> MYVFRFHISSFHSFLVNFLQPSRGVGEPSRLLHHLETHPSYMRRVTSTAVHRTVSSVLSPALLPSFNGTLLLSVCFASCSAAPVRNLYKRLGLDHKATSEEVKAAYRQRALECHPDVVDDNQKAQAEVDFRAVSEAYDVLIDPQKRKEHDKALGLERTVPPAKKQQEGEGVGCDSKGSFNRGVTRPRNRKPFVRGDADRNFREAFHGMSLDQVLFRERLRQRRMQKQMEEKAKEGDDGSPAGREESIRRVAAAAAERFAEKVRRQYGPGMLRHARVYTSLSRDPQPPPSDYMPFRPFHGWTVPNGVRTPPEPTLGPTAKVEDVKDVQLA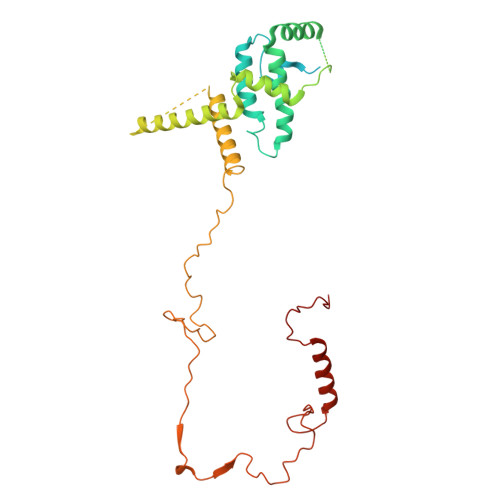EPAVGDASHQRKLPKHFPVVQASDGSSLLREETIACMERERRLPHNMGKLYSYHRPY> TATVLLEVPFSARGDRIPDAVAELRTREPIRKVRTITGAEAWLVSSYALCTQVLEDRRFSMKETAAAGAPRLNALTVPPEVVNNMGNIADAGLRKAVMKAITPKAPGLEQFLRDTANSLLDNLITEGAPADLRNDFADPLATALHCKVLGIPQEDGPKLFRSLSIAFMSSADPIPAAKINWDRDIEYMAGILENPNITTGLMGELSRLRKDPAYSHVSDELFATIGVTFFGAGVISTGSFLTTALISLIQRPQLRNLLHEKPELIPAGVEELLRINLSFADGLPRLATADIQVGDVLVRKGELVLVLLEGANFDPEHFPNPGSIELDRPNPTSHLAFGRGQHFCPGSALGRRHAQIGIEALL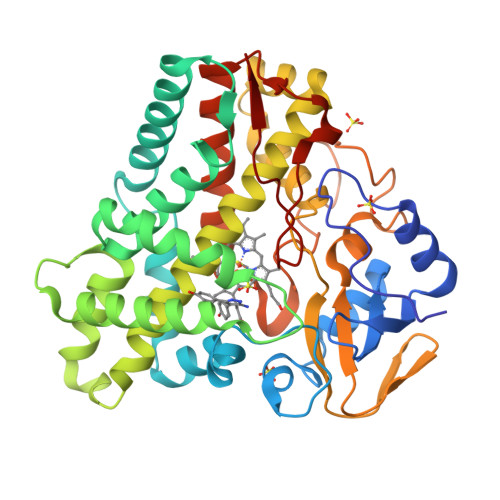KKMPGVDLAVPIDQLVWRTRFQRRIPERLPVLW>VSPIIATILLIAITVVLAATLVTILGGFTHGVSNTVETAGVTSHITSKYIFINVSSSSSAISASSITITITGASFKVTSGDTLAEVAGVSSTSSNATFTGGSDYTVPISLSSSQTVAGVS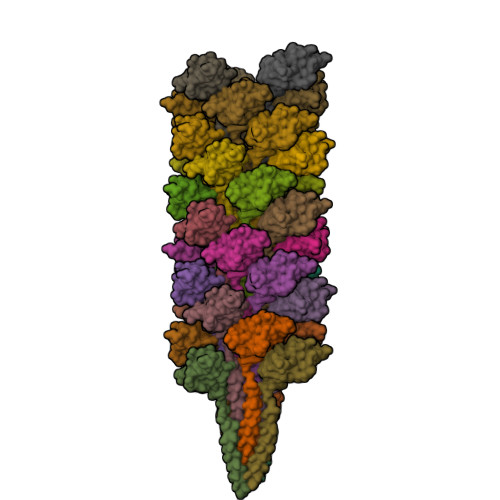FELIYKGNVIYNSAA[36x]>[6x]ATPHNSAQVGDFAETVLMCGDPLRAKLIAETYLENPKLVNNVRGIQGYTGTYKGKPISVMGHGMGLPSICIYAEELYSTYKVKTIIRVGTCGAIDMDIHTRDIVIFTSA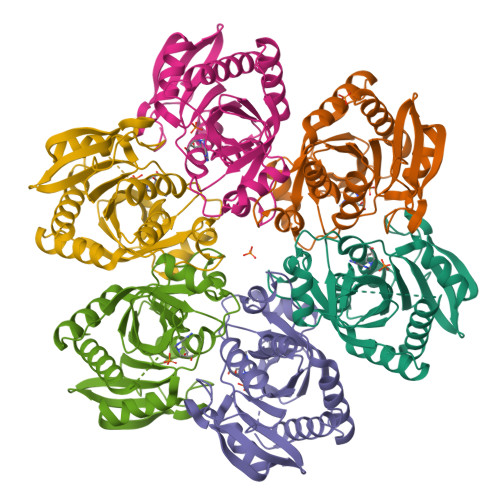GTNSKINRIRFMDHDYPATASFDVVCALVDAAKELNIPAKVGKGFSTDLFYNPQTELAQLMNKFHFLAVEMESAGLFPIADLYGARAGCICTVSDHILHHEETTAEERQNSFQNMMKIALEAAIKLHHHH>[2x]GSVVIVGRIILSGKGGPITAYSQQTRGLLGCIITSLTGRDRNQVEGEVQVVSTATQSFLATCVNGVCWTVYHGAGSKTLAGPKGPITQM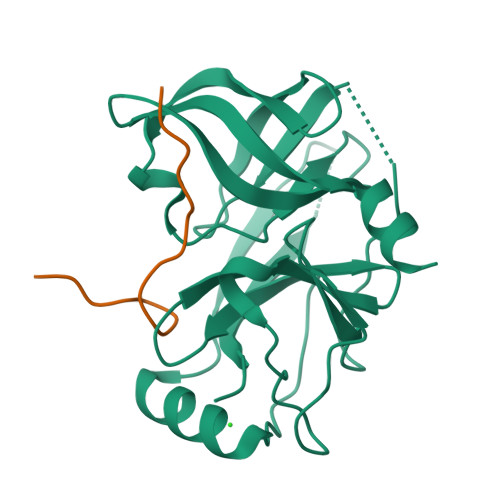YTNVDQDLVGWQAPPGARSLTPCTCGSSDLYLVTRHADVIPVRRRGDSRGSLLSPRPVSYLKGSSGGPLLCPSGHAVGIFRAAVCTRGVAKAVDFVPVESMETTMRGSHHHHHH;>GELDELVYLLDGPGYDPIHS[2x]In this work, we exhaustively probe the ability of all 36 immobile HJ sequences to form DNA crystals in two different designed systems. Three separate self-assembling DNA crystal systems are described in this report: the “4 × 5” and “4 × 6” designs (collectively referred to as the 4 × N systems), and a third construct with a “scrambled” sequence variant of the 4 × 6 lattices. Self-assembly was mediated by three constituent oligonucleotides: (S1) containing four sequence repeats of either 5 or 6 bases; (S2) composed of 21 bases containing complementary regions to both (S1); and (S3) which forms the second junction crossover. The HJ serves as the fundamental component at the core of each unit, and the ultimate assembly of the full lattice is facilitated by the complementary 2-base sticky ends that tail each duplex.

Each asymmetric unit could be defined as either a HJ containing 10 and 11 bp on each arm, or as a 21-bp linear duplex. To investigate this possibility, we designed “scrambled” sequences with targeted base substitutions, while maintaining GC content, along each “stem”. Contrary to the buffer preference observed with the native P32 crystals, the scrambled systems exhibited an exclusive preference towards low salt buffers, much like the native R3 crystals. Remarkably, only J1 and J2 retained the P32 symmetry, with all others yielding an R3 lattice. There appeared to be only a marginal difference in the average cell lengths in the R3 scramble crystals (a = b = 113.04 c = 51.10) relative to the native 4 × 6 sequences: the a, b axis trended ~2 Å shorter and c ~1.3 Å longer, whereas in the J1 and J2 cases, the crystals were in good agreement with the original 4 × 6 motif. The average angles of the R3 and P32 crystals were 61.00° (σ = 1.21) and 58.05° (σ = 1.39), respectively. However, in the majority of the crystal structures reported here, the cacodylate anion indeed fits best into the electron density map of our X-ray structures, due to the presence of sodium cacodylate in the crystallization solution.

> TCGTCT;> GAACGACACAGACGACGACTC;> TCGAGTCG;> GTGTCGT> MAETKSMFREVLPKQGQLYVEDITTMVLCKPKLL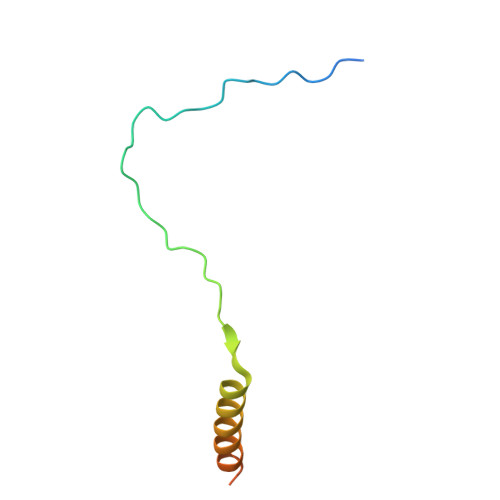PLKSLTLEKLEKMQQAAQDTIHQQEMTEKEQKITH>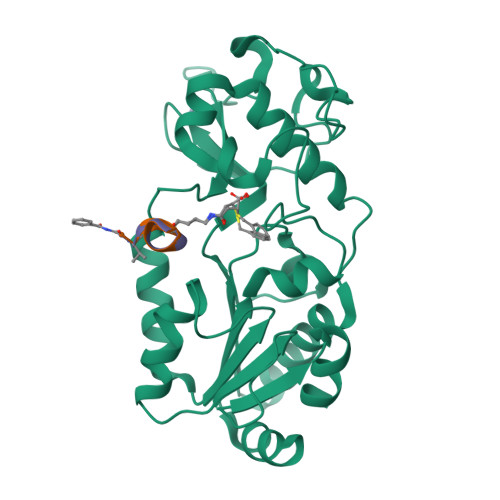[2x]GIDPFTKMTRPSSDLTAFREHFAKAKHIAIITGAGVSAESGVPTFRGPGGFWRKWQAQDLATPEAFSRDPSLVWEFYHYRREVMRSKMPNPAHLAIAECEARLGQQGRSVVIITQNIDELHHRAGSKHVYEIHGSLFKTRCMSCGEVKANHKSPICPALDGKGAPDPNTKEARIPVELLPRCERKSCNGLLRPHVVWFGETLDSDILTAVERELEKCDLCLVVGTSSIVYPAAMFAPQVASRGVPVAEFNMECTPATQRFKYHFEGPCGSTLPPALERHESEAV;>XVLKEYGV[2x]> GSMKNPQSKADDILQCARTLIIRGGYNSFSYADISQVVGIRNASIHHHFPSKSDLVCKLVSQYRQEAEAGIAELEKNISDPLEQLRAYIGYWEGCIADATHPFCVCALLASEIPVLPETVVLEVRAHF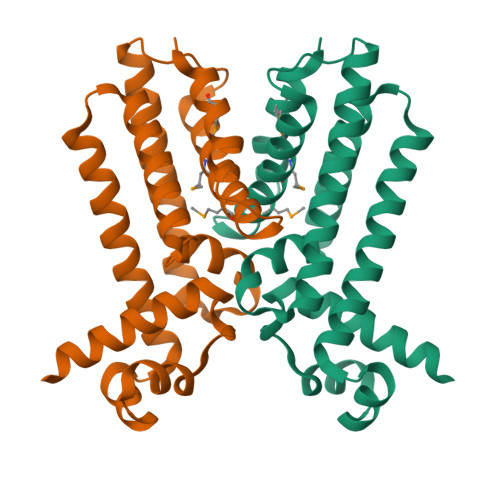RSLSDWLTAVLERGIAQGRLVLTGTARANAEIFMATVHGAMLSARAHGDAATFGAITRPMLERITA4-(acetylamino)-N-[2-amino-5-(thiophen-2-yl)phenyl]benzamide 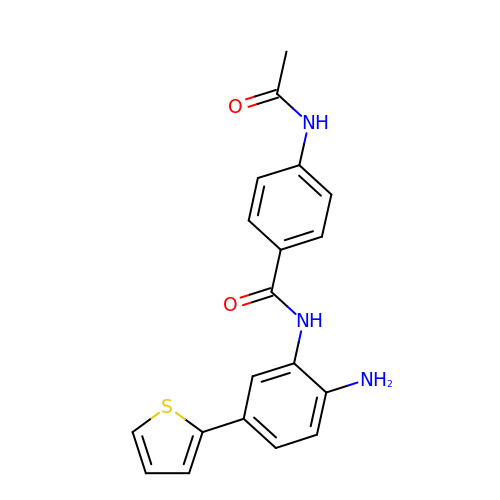| C19 H17 N3 O2 S | ABZSPJVXTTUFAA-UHFFFAOYSA-N> SFKYESAVQYRPAPDSYLNPCPQAGRIVKETYTGINGTKSLNVYLPYGYDPNKKYNIFYLMHGGGENENTIFSNDVKLQNILDHAIMNGELEPLIVVTPTFNGGNCTAQNFYQEFRQNVIPFVESKYSTYAESTTPQGIAASRMHRGFGGFSMGGLTTWYVMVNCLDYVAYFMPLSGDYWYGNSPQDKANSIAEAINRSGLSKREYFVFAATGSEDIAYANMNPQIEAMKALPHFDYTSDFSKGNFYFLVAPGATHWWGYVRHYIYDALPYFFHELEHHHHHH

ID30B is an undulator-based high-intensity, energy-tuneable (6.0–20 keV) and variable-focus (20–200 µm in diameter) macromolecular crystallography (MX) beamline at the ESRF. It was the last of the ESRF Structural Biology Group’s beamlines to be constructed and commissioned as part of the ESRF’s Phase I Upgrade Program and has been in user operation since June 2015. Since its first commissioning experiments, ID30B has proved to be a versatile MX beamline that expands the experimental capabilities of the JSBG beamline portfolio at the ESRF. ESRF beamline ID30B has been in full user operation, including remote access, since June 2015 and, at the time of writing, data collected at the beamline has resulted in 83 PDB depositions and 62 publications.

To further illustrate the capabilities of the beamline, several single-wavelength anomalous diffraction (SAD) experimental phasing measurements were carried out on three test proteins. Diffraction data from a single flash-frozen crystal were collected at 100 K using an X-ray beam size of 30 µm2 with a flux of 2.3 × 1011 photons s−1 at the peak of the Zn K absorption edge (λ = 1.282 Å). Next, a seleno­methione-derivative of the feruloyl esterase module of xylanase 10B from Clostridium thermocellum (FAE) was crystallized and cryoprotected as previously described. Diffraction data from a single flash-frozen crystal were collected at 100 K using an X-ray beam size of 30 µm2 with a flux of 3.3 × 1011 photons s−1 at the peak of the Se K absorption edge (λ = 0.9792 Å). All three structures were then refined using the PDB_redo server and model building carried out in Coot. A summary of all crystallographic information is shown in Table 3.>SPTLEVDALVLNPGRQEASFDGQTLELTGTEFTLLYLLAQHLGQVVSREHLSQEVLGKRLTPFDHAIDMHISNLRRK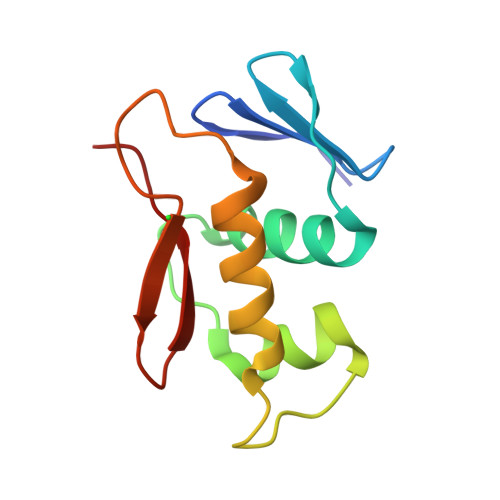LPDRKDGHPWFKTLRGRGYLMVSAA[2x]>MPEGPELHLASQFVNEACRALVFGGCVEKSSVSRNPEVPFESSAYRISASARGKELRLILSPLPGAQPQQEPLALVFRFGMSGSFQLVPREELPRHAHLRFYTAPPGPRLALCFVDIRRFGRWDLGGKWQPGRGPCVLQEYQQFRENVLRNLADKAFDRPICEALLDQRFFNGIGNYLRAEILYRLKIPPFEKARSVLEALQQHRPSPELTLSQKIRTKLQNPDLLELCHSVPKEVVQLGGKGYGSESGEEDFAAFRAWLRCYGMPGMSSLQDRHGRTIWFQGDPGPLAPKGRKS[2x]

Human endonuclease VIII-like 1 (hNEIL1) is a bifunctional DNA glycosylase of the Fpg/Nei family, which catalyzes the removal of damaged bases and subsequent incision of the newly generated abasic sites. Unlike traditional enzymes which are commonly referred to as highly specific biocatalysts, one special feature for hNEIL1 is its unique capability to recognize a wide range of substrates, including formamidopyrimidines, hydantoin lesions, oxidized, and dihydro-modified pyrimidine bases, derived from all four canonical bases. Here, by integrating structural, computational, and biochemical investigations, we show that hNEIL1 uses a triage mechanism to achieve broad specificity and reduce futile repair of normal bases. This mechanism involves two mutually competing interaction states: an activated state that commits catalysis and BER, and a quarantine state that temporarily separates and prevents the flipped base from catalysis via auto-inhibition.

We next performed simulations for hNEIL1(K242)–dT, which prefers damage recognition using the activated state, to examine whether K242 would differentially influence the recognition of a normal dT. We calculated the relative stability of the two competing interaction states for hNEIL1(K242)–dT. Surprisingly, we found that the two states are of similar stability, hinting that dT is more likely to undergo catalysis in the presence of hNEIL1(K242). This observation from simulation was further supported by a new crystal structure, where we found that hNEIL1 adopts the 242-in conformation and that the thymine base is actually removed by hNEIL1(K242) in crystallo. Furthermore, our biochemical data demonstrate that over the course of 72 h, hNEIL1(K242) is capable of cleaving a significantly higher portion of dT than the edited form R242 (using a duplex DNA containing a mismatched T:C pair). Taken together, these results show that the genomically encoded K242 is faster in damage repair but more prone to error, while the edited R242 is slower but safer. In addition, such pre-catalysis checking mechanism also enabled cells to regulate the repair function of hNEIL1, as demonstrated by the RNA editing event that recodes the key residue at position 242: unedited hNEIL1(K242) is faster but riskier in damage repair, while edited hNEIL1(R242) is slower but safer.>QKALDLKDITSGRFRPENIQGVIPMPDGEHYTQMSADGTQIIKYSFRTGEKVEVIFDVNQARECDFKNFDSYQFSPDGDKLLIATRTTPIYRHSYTAVHYIYPLKRNDKGVTTNNIIERLSDGGPQQVPVFSPDGTMIAFVRDNNIFLVKLLYGNSESQVT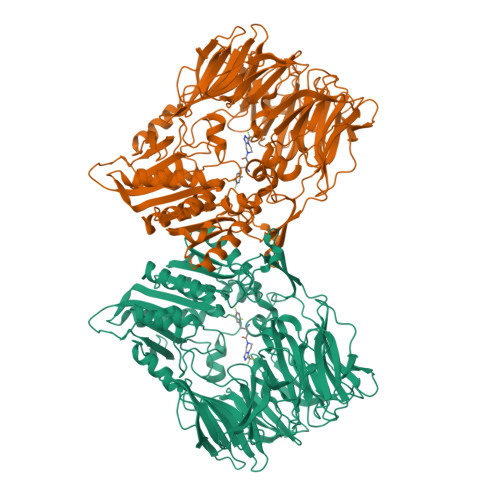EDGKQNSVLNGIPDWVYEEEFGFNRALEFSADNTMIAFIRFDESEVPSYSFPMFAGEAPQITPLKDYPGEYTYKYPKAGYPNSKVEVRTYDIKSHVTRTMKLPIDADGYIPRIRFTKDASKLAVMTLNRHQDRFDLYFADPRSTLCKLVLRDESPYYIKENVFDNIKFYPETFSLLSERDGFSHLYWYSMGGNLIKKVTNGKYEVKDFLGYDEADGSFYYTSNEESPLRKAVYKIDKKGKKLKLSQREGTNTPLFSQSMKYYMNKFSNLDTPMLVTLNDNTGKTLKTLINNDQLKQTLSGYAIPQKEFFTFQTTDGVTLNGWMMKPANFSTSKKYPVLMYQYSGPGSQQVLDTWGISWETYMASLGYIVVCVDGRGTGGRGEAFEKCTYLKIGVKEAKDQVETALYLGKQPYVDKDRIGIWGWSYGGYMTLMSMSEGTPVFKAGVAVAAPTDWRFYDTIYTERFMRTPKENAEGYKESSAFTRADKLHGNLLLVHGMADDNVHFQNCAEYAEHLVQLGKQFDMQVYTNRNHGIYGGNTRQHLYTRLTNFFLNNL[3x]> QRGKNRGCVLTAIHLNVTDLGLGYETKEELIFRYCSGSCDAAETTYDKILKNLSRNRRLVSDKVGQACCRPIAFDD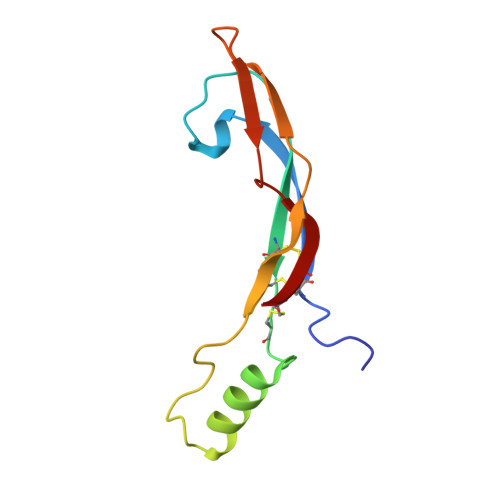DLSFLDDNLVYHILRKHSAKRCGCI> MSMLKREDWYDLTRTTNWTPKYVTENELFPEEMSGARGISMEAWEKYDEPYKITYPEYVSIQREKDSGAYSIKAALERDGFVDRADPGWVSTMQLHFGAIALEEYAASTAEARMARFAKAPGNRNMATFGMMDENRHGQIQLYFPYANVKRSRKWDWAHKAI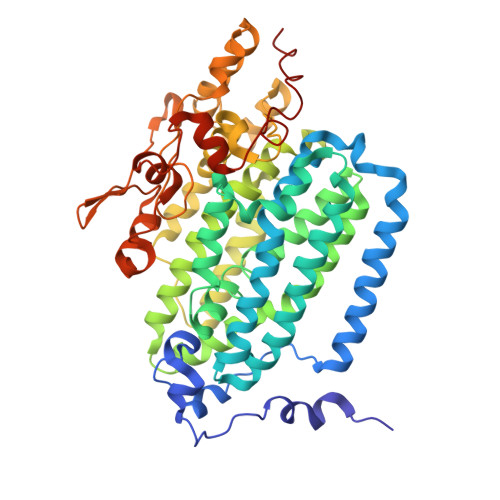HTNEWAAIAARSFFDDMMMTRDSVAVSIMLTFAFETGFSNMQFLGLAADAAEAGDHTFASLISSIQTDESRHAQQGGPSLKILVENGKKDEAQQMVDVAIWRSWKLFSVETGPIMDYYTPLESRNQSFKEFMLEWIVAQFERQLLDLGLDKPWYWDQFMQDLDETHHGMHLGVWYWRPTVWWDPAAGVSPEEREWLEEKYPGWNDTWGQCWDVITDNLVNGKPELTVPETLPTICNMCNLPIAHTPGNKWNVKDYQLEYEGRLYHFGSEADRWCFQIDPERYKNHTNLVDRFLKGEIQPADLAGALMYMSLEPGVMGDDAHDYEWVKAYQKKTNAA>SMDSSALPDPGFQKITLSSSSEEYQKVWNLFNRTLPFYFVQKIERVQNLALWEVYQWQKGQMQKQNGGKAVDERQLF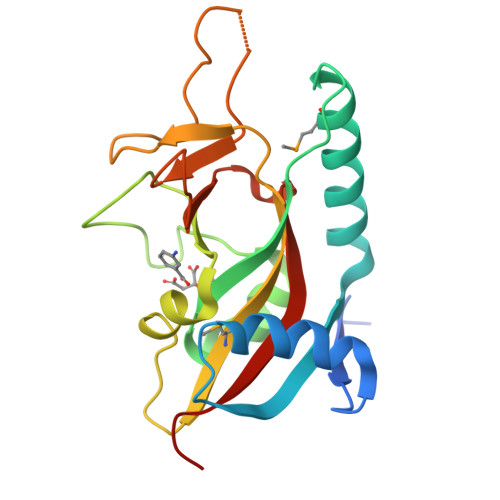HGTSAIFVDAICQQNFDWRVCGVHGTSYGKGSYFARDAAYSHHYSKSDTQTHTMFLARVLVGEFVRGNASFVRPPAKEGWSNAFYDSCVNSVSDPSIFVIFEKHQVYPEYVIQYTTSSKPS[6x]> MSDLGSEELEEEGENDLGEYEGERNEVGERHGHGKARLPNGDTYEGSYEFGKRHGQGTYKFKNGARYTGDYVKNKKHGQGTFIYPDGSRYEGEWADDQRHGQGVYYYVNNDTYTGEWFNHQRHGQGTYLYAETGSKYVGTWVHGQQEGAAELIHLNHRYQGKFMNKNPVGPGKYVFDIGCEQHGEYRLTDTERGEEEEEEETLVNIVPKWKALNITELALWTPTLSEEQPPP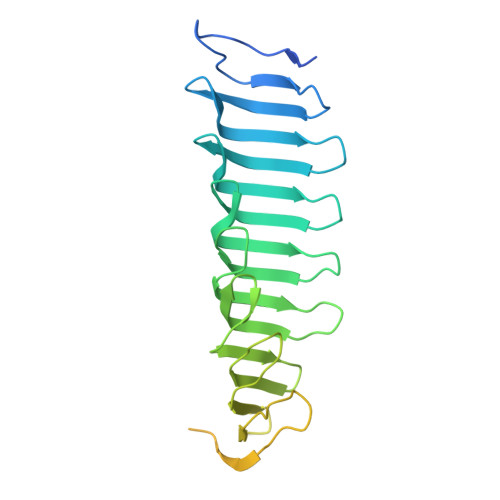EGQGQEEPQGLTGVGDPSEDIQAEGFEGELEPRGADEDVDTFRQESQENSYDIDQGNLNFDEEPSDLQD>MRFVMPGDRIGSAEEYVKGEGVYEEGGELFAAVAGKLIIKDRVAKVESISPIPEIVKGDVVLGRVVDLRNSIALIEVSSKKGENRGPSNRGIGILHVSNVDEGYVKEISEAVGYLDILKARVIGDNLRLSTKEEEMGVLRALCSN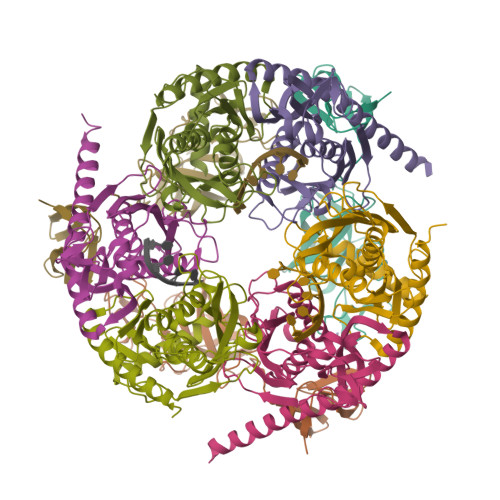CKTEMVREGDILKCPECGRVEKRKISTDYGKGEW[3x];>[3x]MSEFNEKPEKLIVDGLRLDGRKFDELRPIKIEASVLKRADGSCYLEMGKNKVIAAVFGPREVHPEHLQDPSKAIIRYRYNMAPFSVEERKRPGPDRRSIEISKVSKEAFEAVIMKELFPRSAIDIFVEVLQADAGSRTACLNAASVALVDAGVPMKGMITSVAVGKADGQLVLDPMKEEDNFGEADMPFAFLIRNGKIESIALLQMDGRMTRDEVKQAIELAKKGALQIYEMQREAILRRYIEVGEEMDEITEGGEDA;>MPEDILVDIKRDYVLSKLRDNERIDGRGFDEFRKVEIIPNVIEKAEGSALVKLGDTQVVVGVKMQPGEPYPDTPDRGVIIVNAELVPLASPTFEPGPPDENSIELARVVDRGIRESEAVDLSKLVIEEGEKVWIVFVDIHALDDDGNLLDASALAAIAALMNTKVPAERFDLGEDYLLPVRDLPVSVTSLIVGNKYLVDPSREEMSVGDTTLTITTDKDDNVVAMQKSGGYLLDEKLFDELLDVSINCARKLREKFKEI[3x]(2-fluorobiphenyl-4-yl)acetic acid | C14 H11 F O2 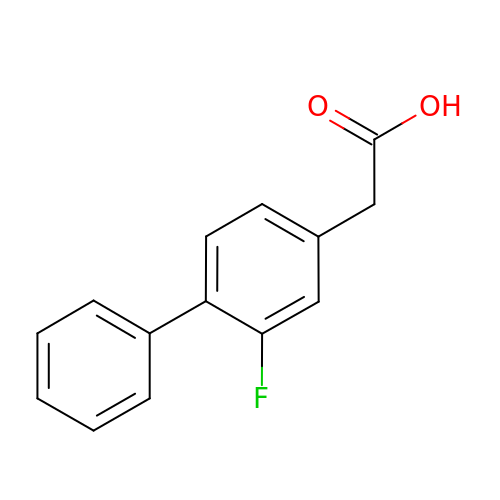| ZLLZRKQQNGBXRD-UHFFFAOYSA-N> MYGSKTFIKYVSGIPDYFKQSFPEGFTWERTTTYEDGGFLTAH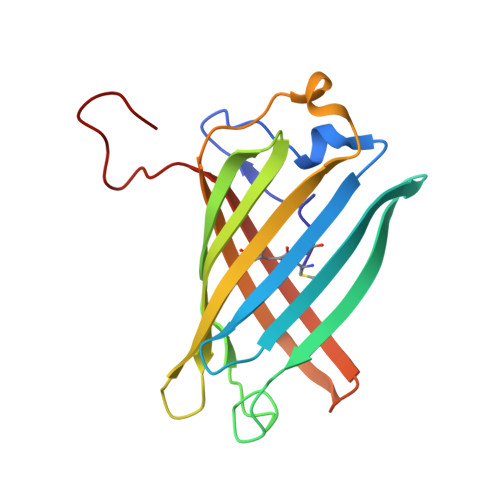QDTSLDGDCLVYKVKILGNNFPADGPVMQNKAGRWEPSTEIVYEVDGVLRGQSLMALKCPGGRHLTCHLHTTYRSKKPASALKMPGFHFEDHRIEIMEEVEKGKCYKQYEAAVGRYCDAAPSKLGHN> MGHHHHHHGSLVPRGSRSRIFKIIVIGDSNVGKTCLTYRFCAGRFPDRTEATIGVDFRERAV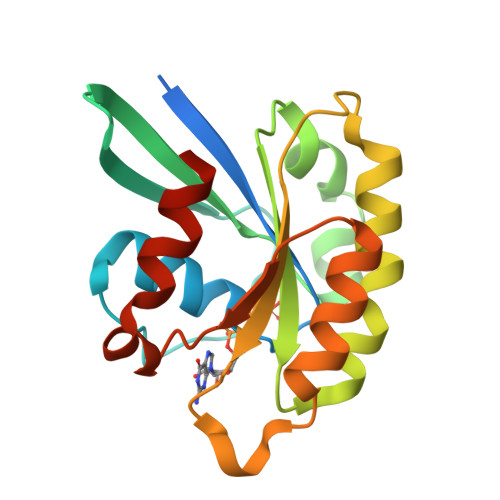DIDGERIKIQLWDTAGQERFRKSMVQHYYRNVHAVVFVYDMTNMASFHSLPAWIEECKQHLLANDIPRILVGNKCDLRSAIQVPTDLAQKFADTHSMPLFETSAKNPNDNDHVEAIFMTLAHKLKSH> MAFDGSIKSLLQGVSQQVPRERLDGQVSVQLNRLSDVVNGNRRRPGARYLADVPTTSQYDDHVFASYVDVQDTANHVIINTETGQLLVISEDFSTTLHNSTQQYLVASAASAIQTATLRGDLYIANTEKAPTKVFGSTTQQDPTKAGFYFVRTPALQKDYDITLSNSTGTYTYTYRTPTGTGTGDADLAKPSYIISDLLAKINAQTGTHGITATAYDAYMFLSSNTVSLSVTTNAGSTYATGSNQSRVSVVSDLPARLPAVGNGASVAVGTTERNFVWYQYDSATSVWKEAGAYGSPTGFSNMPIRISLDGVYTVETPAYEGRLAGSDETNEDPGFIDNGVTGFGAYQGRLVILAGPEVCMSAAGNPLRWYRSTVTALLTDDPINIFSGAATSTNFRHCVQFNKDLLLFARSCQAVVPSSNAAITPQTAQIVITSGYTTDTLAQPGVVGRSVLYSMPRTEHFAGVLEIIPSNTTDSQYTSNDITAHIPRYLPGRIRSIVSSTTSNSSAFICTGDSRSLFIQDYLWSGDEKVQSAWHQWTLPYPIVCTWFVRDRVYIGMRDGTTILVVTIEPQ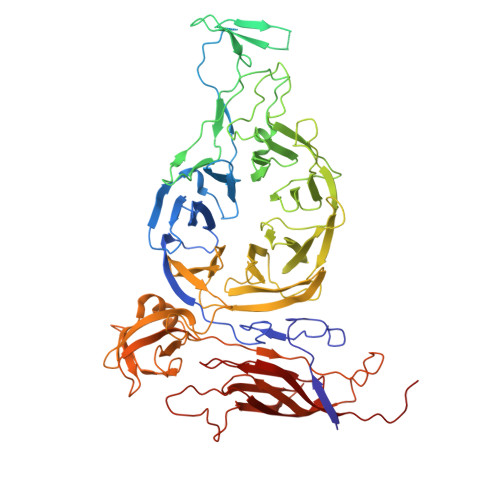AGNTIDSYVRPFSDVYLRVTITDRQFALPTRLRAAVGSGEGLFITFADTSMGGMWVGYESIDPTTYVVTTVRNVPDGEYFVGLRYTSVLSPTPPLVRDANGIVIGTYQSLLVRYELTLKDSGEFHAIITDSSRTLTDGNYSSLVYSSTELLPNNPTDASLGRTIIPVRAQAQDTVATFEANADTDLCILDIEYVLQYRARRKRI> GPGSMSNVAVNTVFASLDNFRKGTVEIISGEARHYAFSNIFEVAQNSKPYEKVVVGLNLGYVVETLRAEGQSPWFTAAHDEFAIVM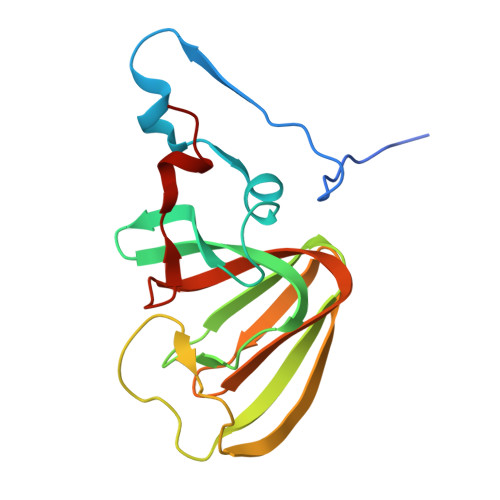DGEVRVEFLKLDAPSKHGEGTHLAGELPVGKPMGYVLLKRGHQCLLPAGSAYRFEASRPGVILQQTIKGPLSVEKWAEICLK> MHHHHHHSSGRENLYFQGSTLSYTLGQLAAHVGAEVRGDADLPIQGLATLQEAGPAQLSFLANPQYRKYLPESRAGAVLLTAADADGFAGTALVVANPYLAYASLSHLFDRKPKAAAGIHPTAIVAADAEVDPSASVGAYAVIESGARIGAGVSIGAHCVIGARSVIGEGGWLAPRVTLYHDVTIGARVSIQSGAVIGGEGFGFANEKGVWQKIAQIGGVTIGDDVEIGANTTIDRGALSDTLIGNGVKLDNQIMIAHNVQIGDHTAMAACVGISGSAKIGRHCMLAGGVGLVGHIEICDNVFVTGMTMVTRSITEPGSYSSGTAMQPAAEWKKSAARIRQLDDMARRLQQLEKRLAAVTSSGDASSD

LpxA and LpxD are functionally and structurally similar, sharing a homotrimer architecture and conserved active site features, especially in the acyl-chain binding pockets that reside in the dimer interface of the β-helix trimer core. Herein we report the discovery of several small molecules that bind to both P. aeruginosa LpxA and LpxD with μM affinity, identified using a targeted structure-based methodology that utilizes molecular docking, surface plasmon resonance (SPR) bioanalysis, and high-resolution X-ray crystallography.

Our LpxD complex structure with compound 1 (2.60 Å) showed distinguishable electron density corresponding to the ligand at the dimer interface formed via crystallographic symmetry. The fitted binding pose suggests that there are two hydrogen bonds stabilizing the protein-ligand complex, both with the backbone nitrogen atoms of two glycine residues, Gly272 and Gly278, from the adjacent monomers forming the active site. Additionally, compound 1 establishes extensive non-polar interactions with residues Ala253, Gly257, Ala271, Leu276, Val277 and Met293, which may also be critical for the hydrophobic contacts with the substrate acyl chain. Compared with the LpxA structure, the ligand’s aromatic ring goes deeper into the LpxD structure, consistent with a slightly larger acyl-chain binding pocket in LpxD. Two conformational changes are observed in LpxD upon ligand binding, one being Ser259. In its apo form, the Ser259 side chain normally points inwards towards the active site. However, the naphthalene ring of compound 1 forces this residue to rotate outwards to avoid steric clash. One of the most interesting observations in the LpxD complex structure is how ligand binding in the acyl-chain binding pocket triggers movement in the distal C-terminal helix, suggesting possible cross-talk between the catalytic pocket and ACP binding site. Our complex structure suggests the possibility of coordination between substrate binding in the active site and ARD binding by ACP. Additionally, there was some residual weak electron density in the active site of LpxD complex crystal with compound 1 suggesting that another ligand copy could possibly be accommodated, although its low occupancy prevented it from being unambiguously identified and modeled at the current resolution.>[2x]MASMTGGQQMGRGSEFMSSLLVKKLVESATTPMRGSEGAAGYDISSVEDVVVPA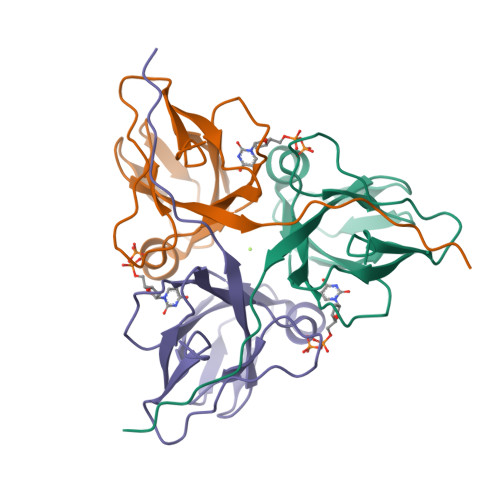MGRIAVSTGISIRVPDGTYGRIAPRSGLAYKYGIDVLAGVIDEDYTGEVKVILYNTTERDYIIKKGDRIAQLILEQIVTPGVAVVLDLSDTARGSGGFGSTGILEHHHHHH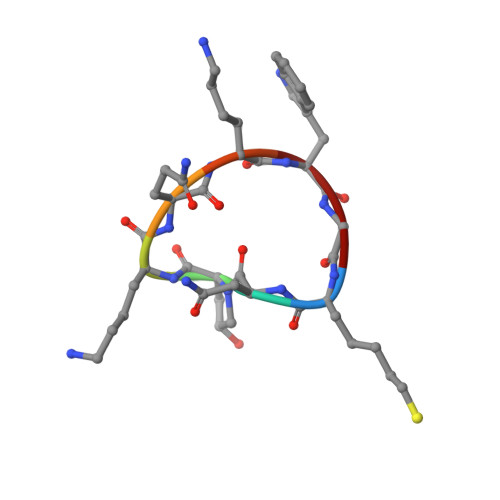> XNPKQKWG>DRHHHHHHKLHWDIFSTWNISLPSVPKPPPKPPSPPAPGAPVSRVLFLTDLHWDHEYLEGTDPYCADPLCCRRGSGWPPNSQKGAGFWGEYSKCDLPLRTLESLLKGLGPAGPFEMVYWTGDIPAHDVWQQSRQDQLRALTTITDLVRKFLGPVPVYPAVGNHESTPVNGFPPPFIKGNQSSQWLYEAMAKAWEPWLPADALHTLRIGGFYALTPRPGLRLISLNMNFCSRENFWLLINSTDPAGQLQWLVEELQAAENRGDKVHIIGHIPPGHCLKSWSWNYYKIIARYENTLAGQFFGHTHVDEFEIFYDEETLSRPLAVAFLAPSATTFINLNPGYRVYQIDGNYPGSSHVVLDHETYILNLTQANAAGGTPSWKRLYRARETY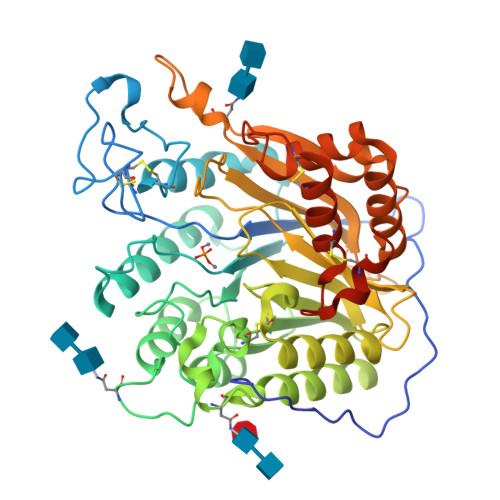GLPDAMPASWHNLVYRMRDDEQLFQTFWFLYHKGHPPSEPCGTPCRLATLCAQLSARADSPALCRHLMPNGSLPDANRLWSRPLLC[2x]>[2x]GTFQFHSPGGKTEIFYDEGERAPVSEIRGEGLTSDSVSLADYKDKIVVLNAWGQW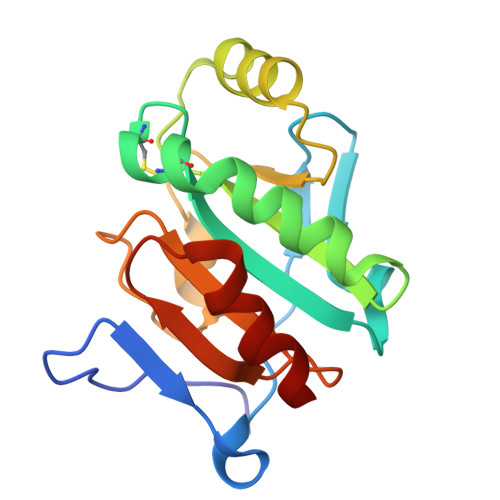CAPCRSESDDLQEVHEYLGDKGTVVGINVRDYSKNIAQDFVKDNGITYPSIYDPPFKTAAQLGGVPASVVPTTIVLDKQHRPAAVFLREVTAQDLIKVIDSLS>MENTENSVASKSIKNLEPKIIHGSESMASGISLDNSYKMDYPEMGLCIIINNKNFHKSTGMTSRSGTDVDAANLRETFRNLKYEVRNKNDLTREEIVELMRDVSKEDHSKRSSFVCVLLSHGEEGIIFGTNGPVDLKKIT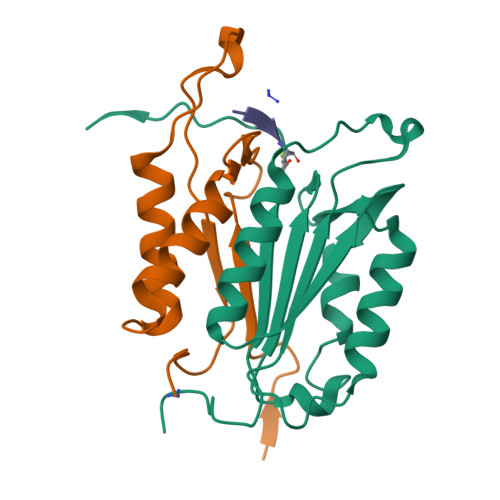NFFRGDRCRDLTGKPKLFIIQACRGTELDCGIETD[2x];>[2x]SGVDDDMACHKIPVEADFLYAYSTAPGYYSWRNSKDGSWFIQSLCAMLKQYADKLEFMHILTRVNRKVATEFESFSFDATFHAKKQIPCIVSMLTKELYFYH> F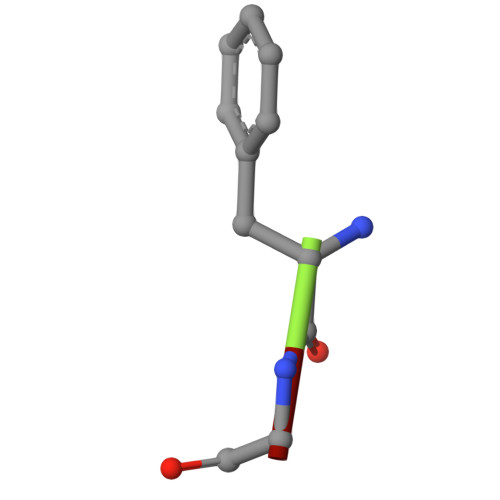GG> MEKSFVITDPRLPDNPIIFASDGFLELTEYSREEILGRNGRFLQGPETDQATVQKIRDAIRDQREITVQLINYTKSGKKFWNLLHLQPMRDQKGELQYFIGVQLDGEFIPNPLLG

miniSOG (for mini Singlet Oxygen Generator)1 is a 106 amino acid flavin-binding protein that generates 1O2 under exposure to blue light. It was originally developed by Shu and coworkers for correlative light and electron microscopy (CLEM) as it both fluoresces and catalyzes the photo-oxidation of diaminobenzidine (DAB), providing high-resolution images. Novel applications are being actively developed since. miniSOG was engineered from the LOV2 (Light, Oxygen and Voltage) domain of Arabidopsis thaliana phototropin 21. The absence of a structure of miniSOG so far had prevented to rationalize these observations, which we have attempted here using a combined structural and photophysical approach.

We have solved the structure of miniSOG at 1.17 Å resolution, which shows an increase in rigidity of the environment of the chromophore compared to that in the LOV2 domain, the location of potential quenchers of the excited states of FMN, and the phosphoribityl tail of FMN lying in a tunnel bridging the bulk solvent and the chromophore encased in the core of the protein. The latter hinders oxygen access to the isoalloxazine ring. 1 ΦΔ=ΦT×kO2kp+kPhot+kO2≈ΦT×kO2kp+kO2 Our structural results above suggest that the low value of kO2 is due to the steric hindrance of the ribityl tail within the tunnel which provides oxygen access to the FMN. Regarding kP, the miniSOG structure shows that six electron-rich residues are positioned within 8.2 to 10.2 Å from the isoalloxazine ring, namely Tyr30, Tyr73, Trp81, His85, Met89 and Tyr98, and are thus close enough to the chromophore to act as electron-transfer quenchers of 3miniSOG*20. In addition, four hydrophilic residues, Glu44, Asp72, Asp82 and Glu103, form hydrogen bonds with FMN, and may thus enhance protein quenching and O2•− formation. Oxygen only quenches 7% of the triplets, which limits Φ∆ to 0.6 × 0.07 = 0.042 (Eq. 1), in excellent agreement with the experimental value. It can therefore be concluded that the modest Φ∆ of miniSOG is due to an unfavorable combination of low kO2 and high kP values, as proposed previously.> EKP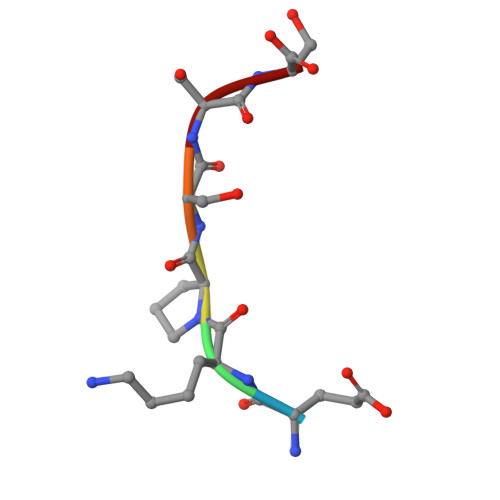SSS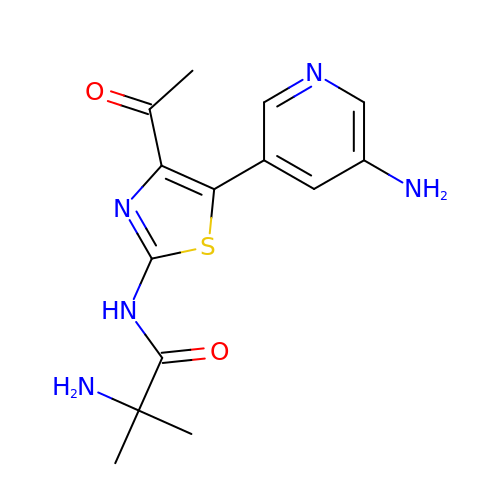2-azanyl-~{N}-[5-(5-azanylpyridin-3-yl)-4-ethanoyl-1,3-thiazol-2-yl]-2-methyl-propanamide | C14 H17 N5 O2 S | FSRJGJACTVPIED-UHFFFAOYSA-N>MASMTGGQQMGRDPMSSIGLAHNVTILGSGETTVVLGHGYGTDQSVWKLLVPYLVDDY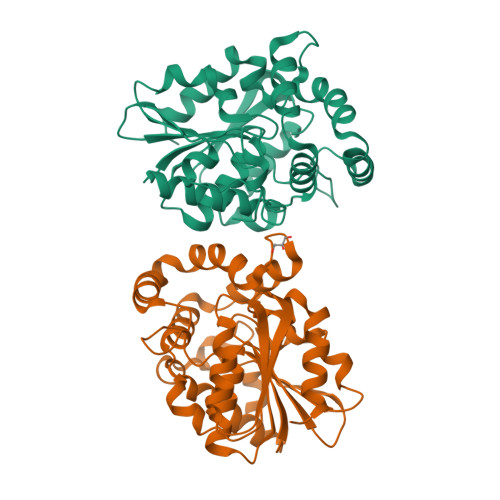KVLLYDHMGAGTTNPDYFDFDRYSSLEGYSYDLIAILEEFQVSKCIYVGHSMSSMAAAVASIFRPDLFHKLVMISPTPRLINTEEYYGGFEQKVMDETLRSLDENFKSLSLGTAPLLLACDLESAAMQEYCRTLFNMRPDIACCITRMICGLDLRPYLGHVTVPCHIIQSSNDIMVPVAVGEYLRKNLGGPSVVEVMPTEGHLPHLSMPEVTIPVVLRHIRQDITDH[2x]Human DDX5 and its yeast ortholog Dbp2 are ATP-dependent RNA helicases that play a key role in normal cell processes, cancer development, and viral infection. Similar to other DEAD-box proteins, DDX5/Dbp2 is composed of two RecA-like domains that include 11 conserved motifs. The helicase core of Dbp2 consists of two RecA-like domains (RecA1: aa 101–319; RecA2: aa 332–465), an NTE (aa 53–100), a CTE (aa 466–496), and a linker (aa 320–331). Here, we report the first X-ray crystal structures of the Dbp2 helicase core alone and in complex with ADP at 3.22 Å and 3.05 Å resolutions, respectively.

The Dbp2 catalytic core bound with ADP (Dbp2-ADP) crystallized in space group P212121 with six molecules (aa 53–496) in the asymmetric unit, arranged in a D3 hexamer. Finally, we obtained the crystal of Dbp2 in complex with ADP and a 16 nt polyGT ssDNA (ssDNA is not visible in the density). When Dbp2 bound to ADP, the two RecA-like domains underwent a large conformational change, distance between the centers of mass of the RecA1-RecA2 domains was reduced to 30.8 Å and the RecA2 domain rotated by 143.9°. Thus, in presence of ADP, the RecA2 domain moved closer to the RecA1 domain and the helicase core adopted a more compact conformation than in the Dbp2-apo structure. Small-angle X-ray scattering (SAXS) analysis showed that Dbp2-ADP is monomeric in solution and the observed hexamer form is probably due to crystal packing. Although the conformation of the helicase core in the crystal structure of Dbp2-ADP was in a semi-closed state, it was in a completely open state in solution. Simultaneously, we observed the interaction of ADP with the Q motif of the RecA1 domain in the Dbp2-ADP structure (blue box). Structural superposition showed that residues R495 and R496 occupy the ADP binding site, and ADP binding resulted in the CTE moving to the side of the RecA2 domain. In the crystal structure of Dbp2-ADP, residue Y221 of the RecA1 domain is close to residues G392 and D393 of the RecA2 domain; therefore, the spatial distance is in favor of an interdomain disulfide bridge formation between the RecA1 and RecA2 domains. Interestingly, the addition of ADP changes the conformation of the helicase core from an open state to a nearly closed state, which is different from the ADP-bound structures of DDX19 (35), DDX21 (36) and Prp5 (34).

>MTYGGRDQQYNKTNYKSRGGDFRGGRNSDRNSYNDRPQGGNYRGGFGGRSNYNQPQELIKPNWDEELPKLPTFEKNFYVEHESVRDRSDSEIAQFRKENEMTISGHDIPKPITTFDEAGFPDYVLNEVKAEGFDKPTGIQCQGWPMALSGRDMVGIAATGSGKTLSYCLPGIVHINAQPLLAPGDGPIVLVLAPTRELAVQIQTECSKFGHSSRIRNTCVYGGVPKSQQIRDLSRGSEIVIATPGRLIDMLEIGKTNLKRVTYLVLDEADRMLDMGFEPQIRKIVDQIRPDRQTLMWSATWPKEVKQLAADYLNDPIQVQVGSLELSASHNITQIVEVVSDFEKRDRLNKYLETASQDNEYKTLIFASTKRMCDDITKYLREDGWPALAIHGDKDQRERDWVLQEFRNGRSPIMVATDVAARGIDVKGINYVINYDMPGNIEDYVHRIGRTGRAGATGTAISFFTEQNKGLGAKLISIMREANQNIPPELLKYDRRSYGGGHPRYGGGRGGRGGYGRRGGYGGGRGGYGGNRQRDGGWGNRGRSNY[6x]> MGDSILSQAEIDALLNGDSDTKDEPTPGIASDSDIRPYDPNTQRRVVRERLQALEIINERFARQ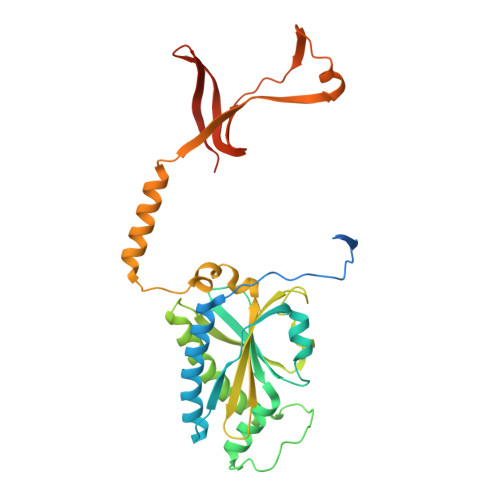FRMGLFNLLRRSPDITVGAIRIQPYHEFARNLPVPTNLNLIHLKPLRGTGLVVFSPSLVFIAVDNLFGGDGRFPTKVEGREFTHTEQRVINRMLKLALEGYSDAWKAINPLEVEYVRSEMQVKFTNITTSPNDIVVNTPFHVEIGNLTGEFNICLPFSMIEPLRELLVNPPLENSRHEDQNWRDNLVRQVQHSELELVANFADIPLRLSQILKLKPGDVLPIEKPDRIIAHVDGVPVLTSQYGTVNGQYALRVEHLINPILNSLNEEQPK CAP is a 210-amino-acid transcription factor that binds cAMP generated by adenylyl cyclase in response to the phosphorylated form of Enzyme IIAGlc (phosphorylated in response to the phosphoenolpyruvate-carbohydrate phosphotransferase system). cAMP-bound CAP regulates the transcription of over 100 genes crucial for carbon utilization through its binding to a specific promoter region and recruitment of RNA polymerase. Previous studies of the ligand binding domain of CAP demonstrated negative cooperativity between cAMP binding sites in the absence of structural change within this domain. We produce coarse-grained models that describe global low-frequency protein backbone motions of CAP and show a strong correlation between negative cooperativity for cAMP and modulation of the delocalised normal modes on ligand binding without a requirement for a spatially distinct physical pathway or conformational change. We demonstrate experimentally that altered connectivity between backbone elements in CAP can give predictable alterations to cooperativity for cAMP binding through altered mode amplitudes.

We therefore used the co-ordinates from a high-resolution crystal structure determination of the full-length cAMP bound CAP homodimer to construct an ENM for the apoprotein as well as single and double ligand bound holoprotein states. The thermodynamic parameters for wild-type CAP demonstrated an overall favourable entropy change and unfavourable enthalpy change on binding the second molecule of cAMP consistent with a previous report. A previous study of the truncated CAP ligand-binding domain demonstrated that binding of the second molecule of cAMP was entropically unfavoured. The difference in thermodynamics between our experiments and previous experiments using the ligand-binding domain alone is therefore likely due to the contribution of motions of the DNA binding domain. The closest distance between the two cAMP molecules in the CAP dimer is 9.5 Å (the distance between the N6 atoms of the adenine ring). The extent of negative cooperativity in CAP is generally small (ΔΔG = 0.3 kcal mol−1). The allostery observed is unlikely to have microheterogeneity as an alternative explanation as all CAP proteins crystallised as a single superimposable structure.

>[2x]MRGSHHHHHHGSMVLGKPQTDPTLEWFLSHCHIHKYPSKSTLIHQGEKAETLYYIVKGSVAVLIKDEEGKEMILSYLNQGDFIGELGLFEEGQERSAWVRAKTACEVAEISYKKFRQLIQVNPDILMRLSAQMARRLQVTSEKVGNLAFLDVTGRIAQTLLNLAKQPDAMTHPDGMQIKITRQEIGQIVGCSRETVGRILKMLEDQNLISAHGKTIVVYGTR We have recently identified interactions between two groups of Drosophila IgSF (immunoglobulin superfamily) cell adhesion molecules with properties closely matching a neuronal chemoaffinity function: 21 Dpr proteins, named after the founding member Defective proboscis extension response, selectively bind nine proteins, now called the Dpr-interacting proteins, or DIPs. All 21 Dprs and nine DIPs are predicted to contain two and three immunoglobulin (IG) domains, respectively. Our previous work identified the first IG domains, termed IG1, as the domains mediating the Dpr–DIP interaction by the formation of a pseudo-symmetric IG1-IG1 heterocomplex using the GFCC’C’ face of the immunoglobulin fold. Therefore, Dprs and DIPs are strong candidates for a synapse specification or targeting function.

As we purified and crystallized several Dpr–DIP complexes, we were also able to grow crystals of DIP-η IG1 and determined its structure at 1.9 Å resolution, which revealed a homodimer. These crystals only grew in the absence of Dpr1, which indicated that the heterodimers are likely more stable than the homodimer under the crystallization conditions used. The homodimeric DIP-η structure closely mimicked the Dpr1–DIP-η heterodimer: When DIP-η monomers were aligned, the other subunits, DIP-η in the homodimer and Dpr1 in the heterodimer, were only displaced by an RMSD of 0.78 Å for 87 out of 102 Cα atoms, excluding the variable DE loop and the mobile half of the A strand. The crystal structures also reveal how DIP-η can accommodate binding to both Dpr1 and itself, with significant differences in sequence at the interface. For example, Tyr103 in Dpr1 (Y, F, or H in Dprs) is replaced by Ile92 in DIP-η (I or V in DIPs). This results in rotameric differences in close-by residue Ile87 in the common DIP-η subunit, which is further accommodated by other rotameric changes in the common DIP-η subunit, and sequence differences between the heterophilic and homophilic partners. The DIP-η homodimers observed in crystals also exist in solution. While size-exclusion chromatography is not an equilibrium experiment, a binding isotherm based on elution peak volumes can be calculated, yielding an apparent KD of 11–45 µM, an order of magnitude weaker than the heterodimer. Furthermore, we performed SPR experiments where low density DIP-η surfaces are created to prevent homodimers on chip surface, and data is fit to a binding isotherm while correcting for DIP-η dimerization in solution, yielding a KD of 14 µM. Here, we also show the presence of DIP-η and DIP-α homodimers in solution and present a symmetrical DIP-η homodimer structure that closely mimics heterodimeric Dpr–DIP complexes.

>SRIVDPKFSSPIVNMTAPVGRDAFLTCVVQDLGPYKVAWLRVDTQTILTIQNHVITKNQRIGIANSEHKTWTMRIKDIKESDKGWYMCQINTDPMKSQMGYLDVVVHHHHHH[2x]> MLPNMRSALKMFEQSVLLKSVETIRVDFVDDIIITATPIRAVVQV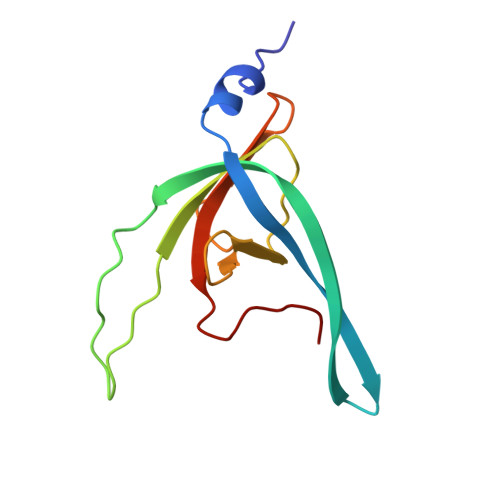ADKKKLNLDSLDWSKQYIWVHSGSKMEIGQFIEWHGKDFKLVAAGDDYSDYGYNAWYGEETLKPVLVSS> GDVEEAIERAVVHVADTMRSGPSNSASVPALTAVETGHTSQVTPSDTMQTRHVKNYHSRSESTVENFLGRSACVYMEEYKTTDNDVNKKFVAWPINTKQMVQMRRKLEMFTYLRFDMEVTFVITSRQDPGTTLAQDMPVLTHQIMYVPPGGPIPAKVDDYAWQTSTNPSIFWTEGNAPARMSIPFISIGNAYSNFYDGWSNFDQRGSYGYNTLNNLGHIYVRHVSGSSPHPITSTIRVYFKPKHTRAWVPRPPRLCQYKKAFSVDFTPTPITDTRKDINTVTTVA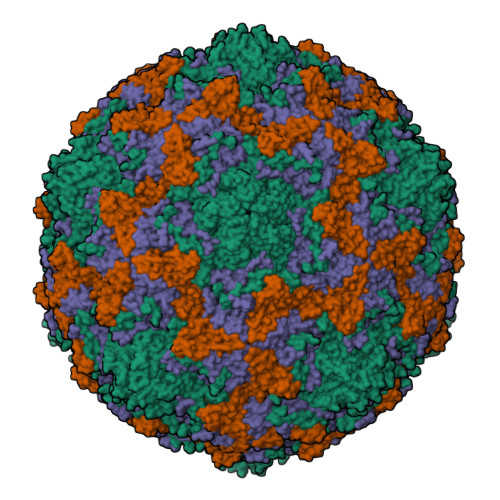QSRRRGDMSTLNTH;> SPTVEECGYSDRVRSITLGNSTITTQECANVVVGYGRWPTYLRDDEATAEDQPTQPDVATCRFYTLDSIKWEKGSVGWWWKFPEALSDMGLFGQNMQYHYLGRAGYTIHVQCNASKFHQGCLLVVCVPEAEMGGAVVGQAFSATAMANGDKAYEFTSATQSDQTKVQTAIHNAGMGVGVGNLTIYPHQWINLRTNNSATIVMPYINSVPMDNMFRHYNFTLMVIPFVKLDYADTASTYVPITVTVAPMCAEYNGLRLAQAQ;> GLPTMNTPGSTQFLTSDDFQSPCALPQFDVTPSMNIPGEVKNLMEIAEVDSVVPVNNVQDTTDQMEMFRIPVTINAPLQQQVFGLRLQPGLDSVFKHTLLGEILNYYAHWSGSMKLTFVFCGSAMATGKFLIAYSPPGANPPKTRKDAMLGTHIIWDIGLQSSCVLCVPWISQTHYRLVQQDEYTSAGYVTCWYQTGMIVPPGTPNSSSIMCFASACNDFSVRMLRDTPFISQDNKLQ;> GAQVSTQKTGAHETSLSAAGNSIIHYTNINYYKDAASNSANRQDFTQDPSKFTEPVKDVMIKSLPALN> GMSQRIGVIDMGTNTFHLLITDIVNDRPHTLVNEKSAVGLGKGGITKGFITEEAMDRALDTLKKFRVILDEHAVVHVIATGTSAVRSGSNKQVLIDRIKKEVNIDVEVIDGAREAELIFRGVQQAVPMEDHISLAMDIGGGSVEFIIGNKNEILWKQSFEIGGQRLIDRFHVHDPMREDDRVMMHNYFDEVLVPLEKAINTWRPTQLIGCSGTFDTLAEMNIQHHREKIALEKQTSYLLSLPDFNR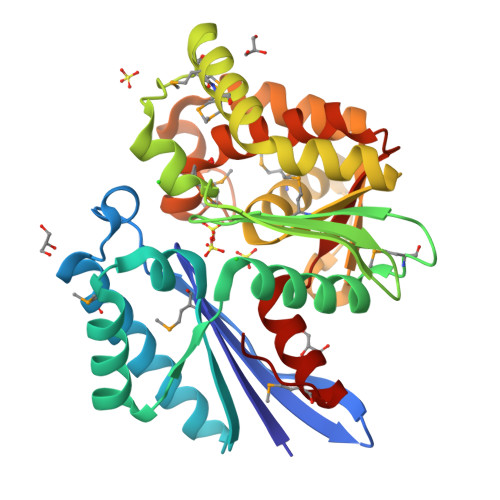LRKQLVASTRRERLAIAGMIELRADMVVVAICLIEHVLKLVSTNAITVSTYSLKEGVLYTMLDGVKVGS Escherichia coli bacteriophage T7, a member of Podoviridae, has been used as a model for understanding the DNA packaging mechanism common to tailed phages and related dsDNA viruses. The phages package genomic dsDNA into a round procapsid using the portal in complex with an ATP-dependent terminase complex as the motor. At the beginning of phage infection, the tail is responsible for receptor recognition, and the portal and tail act as a tunnel for DNA delivery into the host cytoplasm. Here, we determined structures of the DNA packaging intermediate and mature capsids of T7 using cryo-electron microscopy (cryo-EM) and symmetry-mismatch reconstruction.

Another two independent local reconstructions focused on the portal and tail, respectively, yield the structures of the portal and tail at the same resolution of 3.8 Å, suggesting that the portal interacts firmly with the tail. The T7 portal, which exhibits a canonical 12-fold phage portal structure, is formed by 12 copies of the 536-residue portal protein gp8 arranged around a central tunnel. Each gp8 can be divided into five domains of clip (294–334), stem (335–356 and 269–293), wing (1–268, 357–427), crown (428–492), and C-terminal helical barrel. The tunnel is 140 Å in height and of variable tunnel diameter. The narrowest channel is approximately 22 Å in diameter and is formed by a so-called tunnel loop and a long kinked α-helix (α10) in the wing. The 40-Å long C-terminal helical barrel is formed by 12 right-handed twisted α-helices (α13), in stark contrast to the 200-Å long left-handed twisted phage P22 portal helical barrel. An extra rim of the top opening, which is formed by 12 C-terminal α-helices (α14) and loops, interacts with the core. A rod-like density that is approximately 20 Å in diameter and lining the middle of the portal and core channel could be assigned to dsDNA; this is similar to the rod-like density observed in the P22 portal. The dsDNA is embraced by the 12 tunnel loops in the portal, which have a weaker density probably due to its asymmetric interaction with the dsDNA groove. Accordingly, the tunnel loop channel becomes narrower (from 28 to 22 Å in diameter), and the stem channel becomes wider (from 25 to 40 Å in diameter).

>[12x]MAEKRTGLAEDGAKSVYERLKNDRAPYETRAQNCAQYTIPSLFPKDSDNASTDYQTPWQAVGARGLNNLASKLMLALFPMQTWMRLTISEYEAKQLLSDPDGLAKVDEGLSMVERIIMNYIESNSYRVTLFEALKQLVVAGNVLLYLPEPEGSNYNPMKLYRLSSYVVQRDAFGNVLQMVTRDQIAFGALPEDIRKAVEGQGGEKKADETIDVYTHIYLDEDSGEYLRYEEVEGMEVQGSDGTYPKEACPYIPIRMVRLDGESYGRSYIEEYLGDLRSLENLQEAIVKMSMISSKVIGLVNPAGITQPRRLTKAQTGDFVTGRPEDISFLQLEKQADFTVAKAVSDAIEARLSFAFMLNSAVQRTGERVTAEEIRYVASELEDTLGGVYSILSQELQLPLVRVLLKQLQATQQIPELPKEAVEPTISTGLEAIGRGQDLDKLERCVTAWAALAPMRDDPDINLAMIKLRIANAIGIDTSGILLTEEQKQQKMAQQSMQMGMDNGAAALAQGMAAQATASPEAMAAAADSVGLQPGI> MTQAKAKHADVPVNLYRPNAPFIGKVISNEPLVKEGGIGIVQHIKFDLTGGNLKYIEGQSIGIIPPGVDKNGKPEKLRLYSIASTRHGDDVDDKTISLCVRQLEYKHPESGETVYGVCSTYLTHIEPGSEVKITGPVGKEMLLPDDPEANVIMLATGTGIAPMRTYLWRMFKDAERAANPEYQFKGFSWLVFGVPTTPNILYKEELEEIQQKYPDNFRLTYA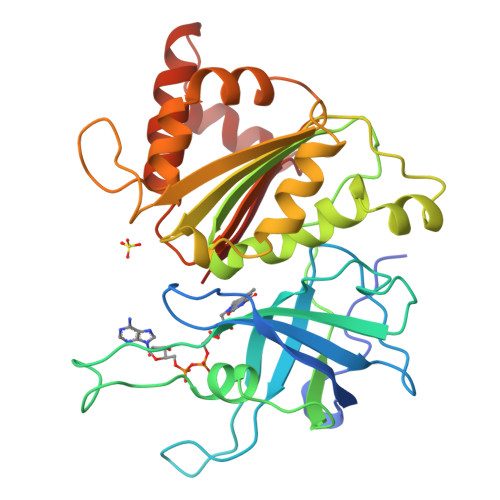ISREQKNPQGGRMYIQDRVAEHADQLWQLIKNQKTHTYICGLRGMEEGIDAALSAAAAKEGVTWSDYQKDLKKAGRWHVATY>[2x]TTNKPIVLSTWNFGLHANVEAWKVLSKGGKALDAVEKGVRLVEDDPTERSVGYGGRPDRDGRVTLDACIMDENYNIGSVACMEHIKNPISVARAVMEKTPHVMLVGDGALEFALSQGFKKENLLTAESEKEWKEWLKTSQYKPIVNIENHNTIGMIALDAQGNLSGACTTSGMAYKMHGRVGDSPIIGAGLFVDNEIGAATATGHGEEVIRTVGTHLVVELMNQGRTPQQACK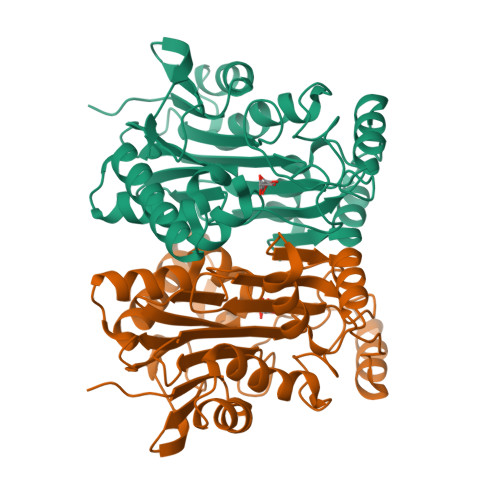EAVERIVKIVNRRGKNLKDIQVGFIALNKKGEYGAYCIQDGFNFAVHDQKGNRLETPGFALK The semaphorins are the largest family of evolutionarily conserved axon guidance cues. The semaphorins signal through their main receptors, plexins, which are single-spanning transmembrane proteins expressed in a variety of cell types, including neurons, cancer cells or endothelial cells. We determined crystal structures of Drosophila Sema1a1–2, Sema1b1–2, Sema2a1–3 and Sema2b1–3 to a 3.6-, 2.8-, 2.1- and 2.5 -Å resolution, respectively. All structures contain the sema domain composed of a seven-bladed β-propeller fold, which is followed by a PSI domain.

The secreted semaphorins Sema2a and Sema2b also contain an Ig-like domain positioned C-terminally to their PSI domains. For example, the Sema2a construct used for crystallization contains eight potential sites for N-linked glycosylation (N95, N163, N190, N229, N314, N401, N563 and N658) and the N-linked glycans were clearly visible and unambiguously fitted into the electron density at N95, N163, N190, N229 (only chain B of the dimer), N314 and N563. Our crystal structures of Drosophila semaphorins revealed that the dimeric architecture in Sema1a, Sema2a and Sema2b is covalently secured by an intermolecular sema-to-sema disulfide bond formed by a cysteine from each of the β4B–β4 C loops of the opposing chains (Cys279 in Sema2a). In the class 2 semaphorins, besides the interchain disulfide bond, dimerization is mediated mainly by the top face of the sema domain using five protruding surface loops, which intertwine with each other to form a massive interface burying a total of 4496 Å2. The Ig-like domain of the class 2 semaphorins is also involved in dimerization and contributes 21% to the total buried surface area of the interface. Remarkably, in the Sema2a structure, an N-linked glycan at residue N314 forms intermolecular interactions with the surface residues of the neighbouring chain. Approximately 17% of the total buried surface area between the two chains of the dimers is contributed by this N-linked glycosylation. The simulations revealed a low inter-domain flexibility that is also obvious from the structural superposition of two independent protein chains observed in Sema2a crystal. The Ig-like domain can reorientate relative to the sema–PSI domains by 14° about a hinge point in the PSI-Ig linker. A superposition of Sema2a1–3 and Sema2b1–3 crystal structures unveiled that Sema2a and Sema2b are also highly similar in structure with an rmsd of 1.1 Å over 608 Cα atoms (for Sema2a chain A and Sema2b chain A).

>ETGYENTWNFYYERPCCTGNDQGNNNYGKHGADHVREFNCGKLYYRTFHMNEDRDTLYVGAMDRVFRVNLQNISSSNCNRDVINLEPTRDDVVSCVSKGKSQIFDCKNHVRVIQSMDQGDRLYVCGTNAHNPKDYVIYANLTYLPRSEYVIGVGLGIAKCPYDPLDNSTAIYVENGNPGGLPGLYSGTNAEFTKADTVIFRTDLYNTSAKRLEYKFKRTLKYDSKWLDKPNFVGSFDIGEYVYFFFRETAVEYINCGKAVYSRIARVCKKDVGGKNLLAHNWATYLKARLNCSISGEFPFYFNEIQSVYQLPSDKSRFFATFTTSTNGLIGSAVCSFHINEIQAAFNGKFKEQSSSNSAWLPVLNSRVPEPRPGTCVNDTSNLPDTVLNFIRSHPLMDKAVNHEHNNPVYYKRDLVFTKLVVDKIRIDILNQEYIVYYVGTNLGRIYKIVQYYRNGESLSKLLDIFEVAPNEAIQVMEISQTRKSLYIGTDHRIKQIDLAMCNRRYDNCFRCVRDPYCGWDKEANTCRPYELDLLQDVANETSDICDSSVLKKKIVVTYGQSVHLGCFVKIPEVLKNEQVTWYHHSKDKGRYEIRYSPTKYIETTERGLVVVSVNEADGGRYDCHLGGSLLCSYNITVDAHRCTPPNKGTKHHHHHH[2x]> MPSELTPEERSELKNSIAEFHTYQLDPGSCSSLHAQRIHAPPELVWSIVRRFDKPQTYRHFIKSCSVEQNFEMRVGCTRDIIVISGLPANTSTERLDILDDERRVTGASIIGGEHRLTNYKSVTTVHRFEKENRIWTVVLESYVVDMPEGNSEDDTRMLADTVVKLNLQKLATVAEAMARN;> GAMGRSVYELDCIPLWGTVSIQGNRSEMEDAFAVSPHFLKLPIKMLMGDHEGMSPSLTHLTGHFFGVYDGHGGHKVADYCRDRLHFALAEEIERIKDELCKRNTGEGRQVQWDKVFTSCFLTVDGEIEGKIGRAVVGSSDK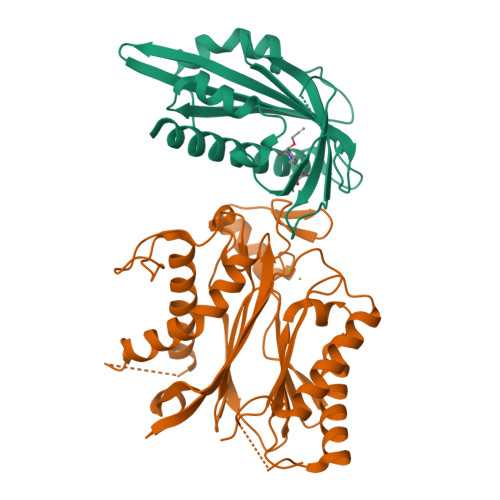VLEAVASETVGSTAVVALVCSSHIVVSNCGDSRAVLFRGKEAMPLSVDHKPDREDEYARIENAGGKVIQWQGARVFGVLAMSRSIGDRYLKPYVIPEPEVTFMPRSREDECLILASDGLWDVMNNQEVCEIARRRILMWHKKNGAPPLAERGKGIDPACQAAADYLSMLALQKGSKDNISIIVIDLKAQR> IS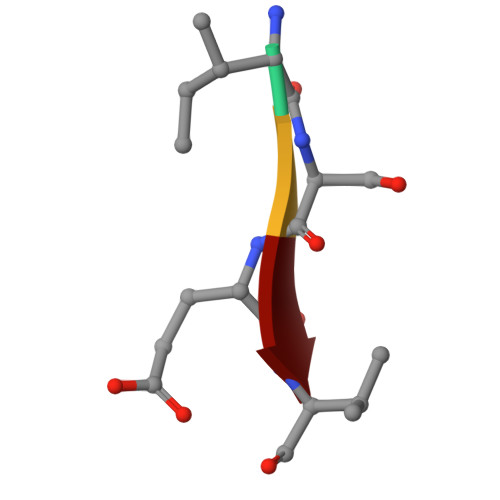EV> SMESVVTVYSIDGLHDGDNSWY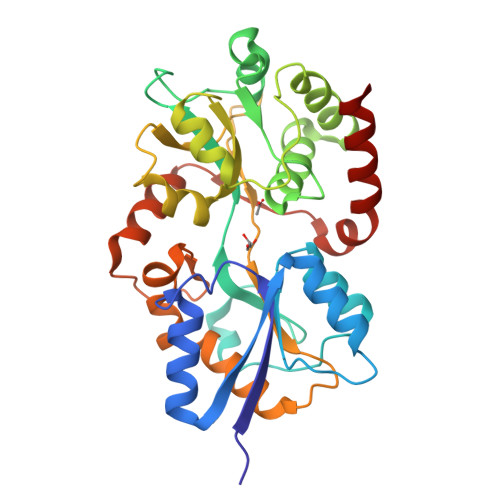QVQFDAFTKATGITVRYVEGGGGVVVERLAKERTNPQADVLVTAPPFIQRAAAEKLLANFNTDTASAIPDANNLYSPLVKNYLSFIYNSKLLKTAPASWQDLLDGKFKNKLQYSTPGQAADGTAVMLQAFHSFGSKDAGFAYLGKLQANNVGPSASTGKLTALVNKGEIYVANGDLQMNLAQMERNPNVKIFWPANDKGERSALAIPYVIGLVQGAPQSENGKKLINFLLSKEAQTRVSELSWGMPVRSDVTPSDEHYKAATAALEGVQSWQPNWDDVAVSLSADISRWHKVTESE> SRIWQSPRF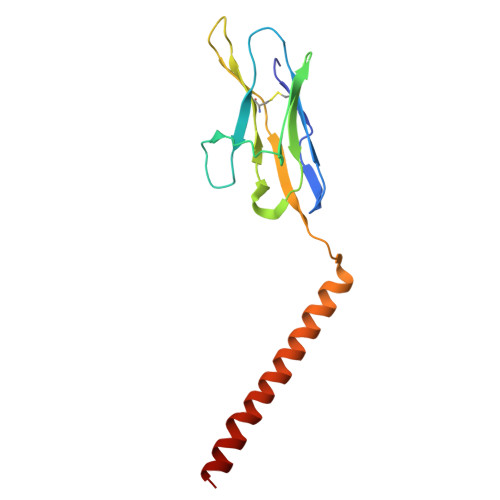IARKRGFTVKMHCYMNSASGNVSWLWKQEMDENPQQLKLEKGRMEESQNESLATLTIQGIRFEDNGIYFCQQKCNNTSEVYQGCGTELRVMGFSTLAQLKQRNTLKDGIIMIQTLLIILFIIVPIFLLLD[[(2R,3S,4R,5R)-5-(6-aminopurin-9-yl)-4-oxidanyl-3-phosphonooxy-oxolan-2-yl]methoxy-oxidanyl-phosphoryl] [(3R)-2,2-dimethyl-3-oxidanyl-4-oxidanylidene-4-[[3-oxidanylidene-3-[2-[(2R)-2-oxidanylundecyl]sulfanylethylamino]propyl]amino]butyl] hydrogen phosphate | C32 H58 N7 O17 P3 S | 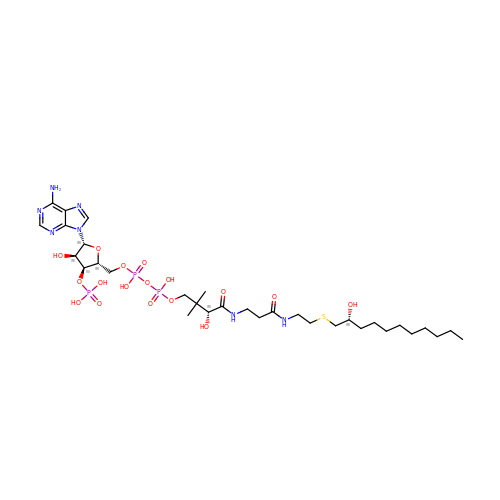LVZITIAGAKKXBV-XBRBJHMKSA-N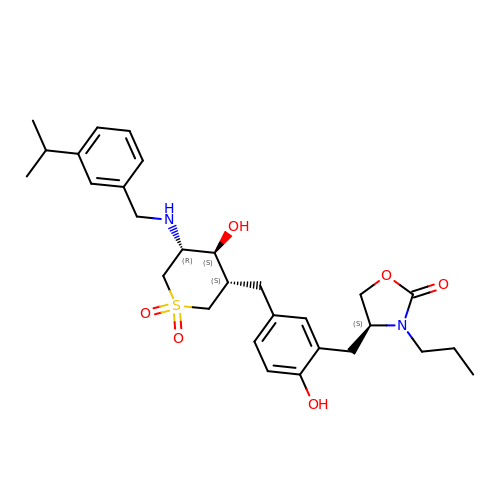(4S)-4-(2-hydroxy-5-{[(3S,4S,5R)-4-hydroxy-1,1-dioxido-5-{[3-(propan-2-yl)benzyl]amino}tetrahydro-2H-thiopyran-3-yl]methyl}benzyl)-3-propyl-1,3-oxazolidin-2-one | C29 H40 N2 O6 S | JYNDAPHZRSRSGI-KAHNYGAISA-N> MGHHHHHHHHHHSSGHIEGRHMLRERTVRLQYGSRVEAVYVLGTYLWTDVYSAAPAGAQTFSLKHSEHVWVEVVRDGEAEEVATNGKQRWLLSPSTTLRVTMSQASTEASSDKVTVNYYDEEGSIPIDQAGLFLTAIEISLDVDADRDGVVEKNNPKKASWTWGPEGQGAILLVNCDRETPWLPKEDCRDEKVYSKEDLKDMSQMILRTKGPDRLPAGYEIVLYISMSDSDKVGVFYVENPAAGQRYIHILGRRKLYHVVKYTGGSAELLFFVEGLCFPDEGFSGLVSIHVSLLEYMAQDIPLTPIFTDTVIFRIAPWIMTPNILPPVSVFVCCMKDNYLFLKEVKNLVEKTNCELKVCFQYLNRGDRWIQDEIEFGYIEAPHKGFPVVLDSPRDGNLKDFPVKELLGPDFGYVTREPLFESVTSLDSFGNLEVSPPVTVNGKTYPLGRILIGSSFPLSGGRRMTKVVRDFLKAQQVQAPVELYSDWLTVGHVDEFMSFVPIPGTKKFLLLMASTSACYKLFREKQKDGHGEAIMFKGLGGMSSKRITINKILSNESLVQENLYFQRCLDWNRDILKKELGLTEQDIIDLPALFKMDEDHRARAFFPNMVNMIVLDKDLGIPKPFGPQVEEECCLEMHVRGLLEPLGLECTFIDDISAYHKFLGEVHCGTNVRRKPFTFKWWH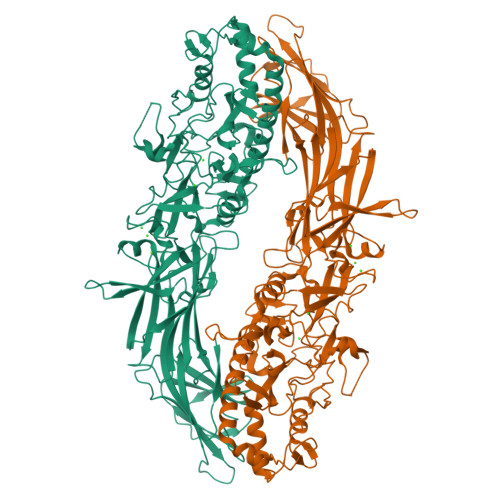MVPSRRS5,5-dihydroxy-6-oxo-L-norleucine 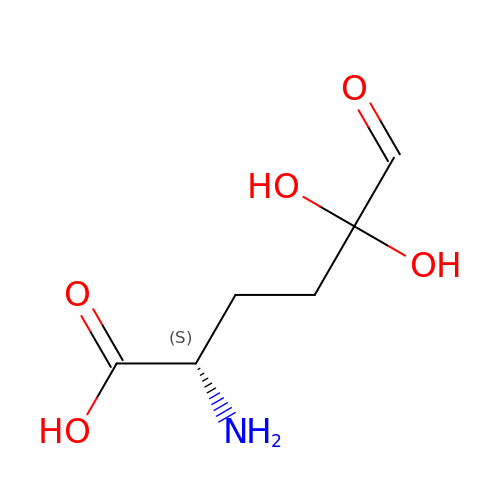| C6 H11 N O5 | GRXWCZHHLRJOLV-BYPYZUCNSA-N> MGSAGKAAEERGLPKGATPQDTSGLQDRLFSSESDNSLYFTYSGQPNTLEVRDLNYQVDLASQVPWFEQLAQFKMPWTSPSCQNSCELGIQNLSFKVRSGQMLAIIGSSGCGRASLLDVITGRGHGGKIKSGQIWINGQPSSPQLVRKCVAHVRQHNQLLPNLTVRETLAFIAQMRLPRTFSQAQRDKRVEDVIAELRLRQCADTRVGNMYVRGLSGGERRRVSIGVQLLWNPGILILDEPTSGLDSFTAHNLVKTLSRLAKGNRLVLISLHQPRSDIFRLFDLVLLMTSGTPIYLGAAQHMVQYFTAIGYPCPRYSNPADFYVDLTSIDRRSREQELATREKAQSLAALFLEKVRDLDDFLWKAETKDLDEDTCVESSVTPLDTNCLPSPTKMPGAVQQFTTLIRRQISNDFRDLPTLLIHGAEACLMSMTIGFLYFGHGSIQLSFMDTAALLFMIGALIPFNVILDVISKCYSERAMLYYELEDGLYTTGPYFFAKILGELPEHCAYIIIYGMPTYWLANLRPGLQPFLLHFLLVWLVVFCCRIMALAAAALLPTFHMASFFSNALYNSFYLAGGFMINLSSLWTVPAWISKVSFL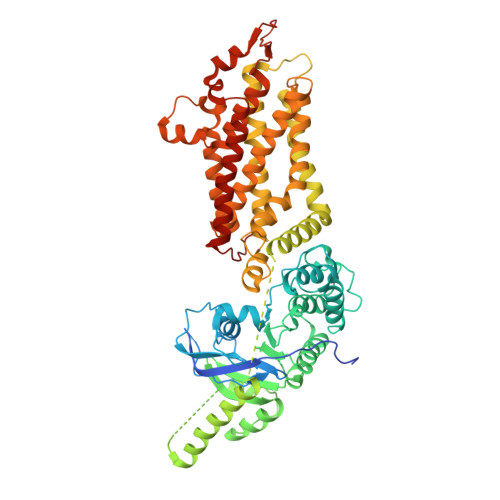RWCFEGLMKIQFSRRTYKMPLGNLTIAVSGDKILSVMELDSYPLYAIYLIVIGLSGGFMVLYYVSLRFIKQKPSQDWASNSLEVLFQ> GPTAAALETAVYSKSGGLLPEPHRTSFGIIRLILTVVPGLLIGAAISKNIANFL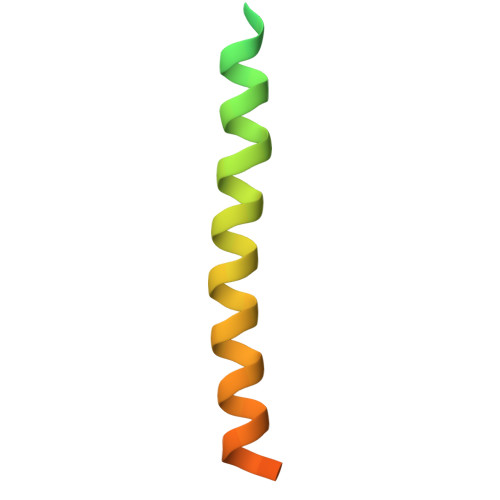EENDLFVPSDDDDDDD HYPOPHOSPHITE 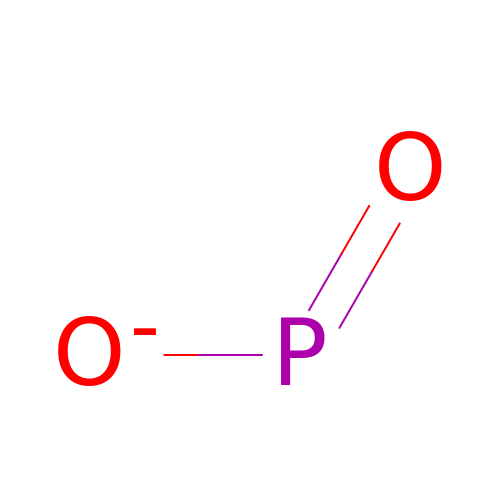| O2 P | GQZXNSPRSGFJLY-UHFFFAOYSA-M> GSHKKLVVKVHMDDSSTKSLMVDERQLARDVLDNLFEKTHCDCNVDWCLYEIYPELQIERVFEDHENVVEVLSDWTRDTENKVLFLEKEERYAVFKNPQNFYLDNKGKKENKETNEKMNAKNKEYLL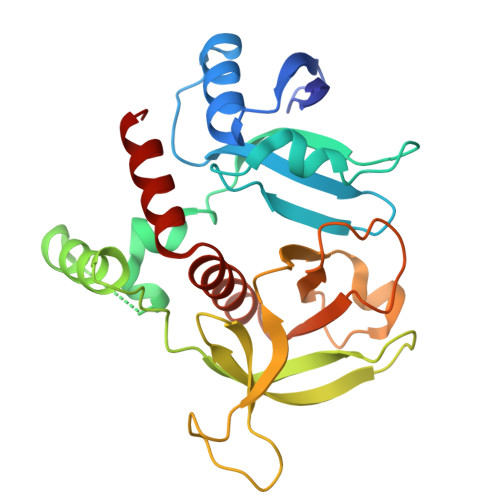EESFCGTSIIVPELEGALYLKEDGKKSWKRRYFLLRASGIYYVPKGKTKTSRDLACFIQFENVNIYYGIQCKMKYKAPTDHCFVLKHPQIQKESQYIKYLCCDDARTLSQWVMGIRIAKYGKTLYDNYQRAVARA>LTAKHRPSVVWLHNAECTGCTEAAIRTIKPYIDALILDTISLDYQETIMAAAGEAAEAALHQALEGKDGYYLVVEGGLPTIDGGQWGMVAGHPMIETTKKAAAKAKGIICIGTCSAYGGVQKAKPNPSQAKGVSEALGVKTINIPGCPPNPINFVGAVVHVLTKGIPDLDENGRPKLFYGELVHDNCPRLPHFEASEFAPSFDSEEAKKGFCLYELGCKGPVTYNNCPKVLFNQVNWPVQAGHPCLGCSEPDFWDTMTPFYEQG[3x];>[3x]MAESKPTPQSTFTGPIVVDPITRIEGHLRIMVEVENGKVKDAWSSSQLFRGLEIILKGRDPRDAQHFTQRACGVCTYVHALASSRCVDDAVKVSIPANARMMRNLVMASQYLHDHLVHFYHLHALDWVDVTAALKADPNKAAKLAASIAPARPGNSAKALKAVQDKLKAFVESGQLGIFTNAYFLGGHKAYYLPPEVDLIATAHYLEALHMQVKAASAMAILGGKNPHTQFTVVGGCSNYQGLTKDPLANYLALSKEVCQFVNECYIPDLLAVAGFYKDWGGIGGTSNYLAFGEFATDDSSPEKHLATSQFPSGVITGRDLGKVDNVDLGAIYEDVKYSWYAPGGDGKHPYDGVTDPKYTKLDDKDHYSWM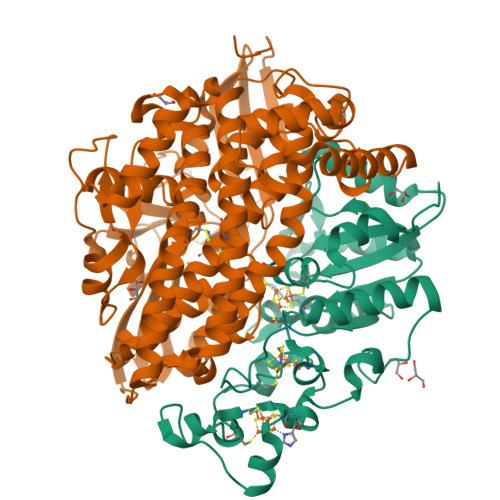KAPRYKGKAMEVGPLARTFIAYAKGQPDFKKVVDMVLGKLSVPATALHSTLGRTAARGIETAIVCANMEKWIKEMADSGAKDNTLCAKWEMPEESKGVGLADAPRGALSHWIRIKGKKIDNFQLVVPSTWNLGPRGAQGDKSPVEEALIGTPIADPKRPVEILRTVHAFDPCIACGVH Human ornithine δ-aminotransferase (hOAT; EC2.6.1.13), which belongs to the same evolutionary subgroup as GABA-AT, converts L-ornithine (L-Orn) into L-glutamate-γ-semialdehyde (L-GSA) while also producing L-Glu from α-KG. Aminotransferases are members of the pyridoxal 5′-phosphate (PLP)-dependent class of enzymes. The PLP moiety links to a catalytic lysine (Lys) residue through a Schiff base, forming an internal PLP–Lys aldimine structure, which can specifically react with an amino acid substrate to produce a keto analog while forming pyridoxamine 5′-phosphate (PMP), thereby completing the first transamination reaction. Consequently, hOAT has emerged as a potential target for developing effective treatments for different types of cancers; therefore, we are interested in determining the mechanistic differences among compounds that inactivate both GABA-AT and hOAT for the future design of selective inactivators of either GABA-AT or hOAT as potential therapeutics.

We further carried out co-crystallization experiments to explore the final product of 5 in hOAT. The acquired crystals diffracted to a resolution of 1.91 Å. The most well refined molecular model had three monomers in an asymmetric unit in the C121 space group. The biological assembly of hOAT is a homodimer. In contrast, the apo-hOAT peak is the primary one in the sample treated with 5, while only a small portion of hOAT was covalently modified by 5 (middle). The conjugated structure of the noncovalent form explains the maximum absorbance at 460 nm. It should also be noted that the carboxylate group forms salt bridges with Arg413 and hydrogen bonds with Gln266 rather than interacting with Arg180 or Tyr55. In the case of noncovalent inhibition by 5, the ligand is located 2.8 Å away from Lys292, resulting in the additional translational freedom for the carboxylate group to anchor with Arg413. The unique binding orientation of 5 also led to a water-mediated hydrogen bond interaction between the imine group of the ligand and Tyr55 residue. The co-crystal complex also reveals for the first time that, in both the minor covalent and major noncovalent forms, the carboxylate group of 5 establishes unusual salt bridges with Arg413 rather than salt bridges with Arg180/Tyr55, as was previously observed in all the co-crystals of hOAT with other MBIs.

>[3x]GPPTSDDIFEREYKYGAHNYHPLPVALERGKGIYLWDVEGRKYFDFLSSYSAVNQGHCHPKIVNALKSQVDKLTLTSRAFYNNVLGEYEEYITKLFNYHKVLPMNTGVEAGETACKLARKWGYTVKGIQKYKAKIVFAAGNFWGRTLSAISSSTDPTSYDGFGPFMPGFDIIPYNDLPALERALQDPNVAAFMVEPIQGEAGVVVPDPGYLMGVRELCTRHQVLFIADEIQTGLARTGRWLAVDYENVRPDIVLLGKALSGGLYPVSAVLCDDDIMLTIKPGEHGSTYGGNPLGCRVAIAALEVLEEENLAENADKLGIILRNELMKLPSDVVTAVRGKGLLNAIVIKETKDWDAWKVCLRLRDNGLLAKPTHGDIIRFAPPLVIKEDELRESIEIINKTILSF> RIIYDRK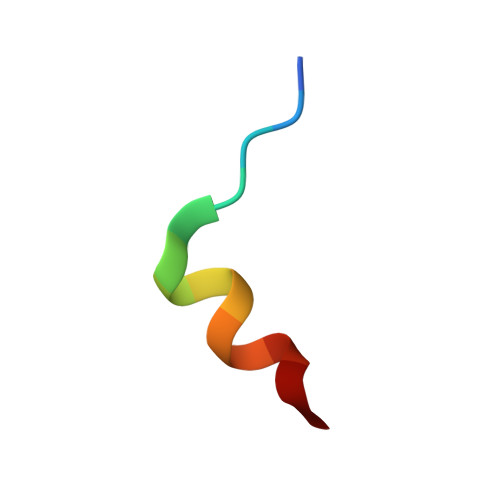FLMECRN>[2x]GMGKRILLLEKERNLAHFLSLELQKEQYRVDLVEEGQKALSMALQTDYDLILLNVNLGDMMAQDFAEKLSRTKPASVIMILDHWEDLQEELEVVQRFAVSYIYKPVLIENLVARISAIFRGRDFIDQHSSLMKVPRTYRNLRIDVEHHTVYRGEEMIALTRREYDLLATLMGSKKVLTREQLLESVWKYESATETNIVDVYIRYLRSKLDVKGQKSYIKTVRGVGYTMQEG

Here we describe the two-component-like orphan response regulator RitR (Repressor of iron transport Regulator) as the archetype of a novel family of peroxide-sensing transcription factors in the pneumococcus and related species. RitR contains an Aspartate-less Receiver (ALR) REC-like domain, which retains the common (α/β) fold of canonical REC versions, yet lacks “invariant” residues in its catalytic pocket required for typical phosphotransfer, including the phospho-accepting Asp residue crucial for the histidine kinase-response regulator phosphorelay.. Here we show that RitR regulates pneumococcal iron homeostasis in response to cellular peroxide concentrations through its single Cys (Cys128) located within the linker domain of the protein. Atomic structures of RitR in its oxidized and reduced states demonstrate a dramatic mechanism of activation that hinges on the helical unraveling and subsequent formation of an inter-protomer disulfide bridge to enable DNA binding and transcriptional regulation of Piu.

The X-ray crystal structure of the full-length reduced state mimic RitRC128S was determined to 1.7 Å resolution with selenomethionine (Se-Met) Single Wavelength Anomalous Diffraction (SAD) method. Thus, to eliminate any heterogeneity caused by this phenomenon, we mutated the redox-active cysteine residue (Cys128) to serine, which would be unable to oxidize and activate the protein. The resulting RitRC128S exhibited no evidence of dimerization in solution using both SEC and 2-dimensional nuclear magnetic resonance (NMR) techniques. The RitRC128S (Se-Met) mutant crystallized in space group C2 with two molecules in the asymmetric unit. These molecules are nearly identical with root mean square deviations of 0.69 Å for all Cα atoms, are independent, and do not form a dimer with each other, nor with any symmetry-related molecule. However, more positive charges are visibly present in PhoB, as RitR contains several aromatic amino acids in these same positions, which are also (notably) able to hydrogen bond with DNA. Finally, we observe that the trans-activation loop (colored magenta in Fig 3), responsible for the binding and direct recruitment of RNA polymerase, would be inaccessible to RNAP in the RitRC128S structure. Combined with the fact that RitR requires oxidation to bind and repress Piu transcription, from these studies we can be fairly confident that the RitRC128S structure is reflective of the inactive, reduced state. The most unique and striking feature of the RitRC128S structure is the α5 helix linker, which connects the REC and DBD sections of the protein.>[2x]MRSVASDREVRGPASTEEELSAVLTSIDSSAIASNIQHHADFTPLFSPEHSSPLKAYHATAKSVFDSLIMNWNATYDYYNKVNAKQAYYLSMEFLQGRALTNAIGNLELTGQYAEALKQLGHNLEDVASQEPDPALGNGGLGRLASCFLDSLATLNYPAWGYGLRYRYGLFKQIITKDGQEEVAENWLEMGNPWEIVRNDVSYPVKFYGKVVEGTDGRKHWIGGENIKAVAHDVPIPGYKTKTTNNLRLWSTTVPSQNFDLGA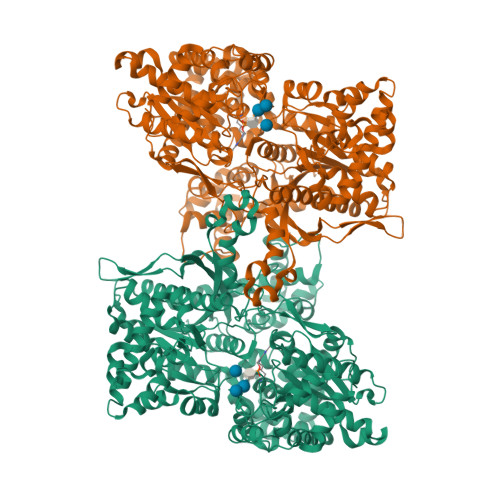FNAGDHAKANEAHLNAEKICHVLYPGDESSEGKILRLKQQYTLCSASLQDIISRFESRAGDSLNWEDFPSKVAVQMNDTHPTLCIPELMRILMDIKGLSWNEAWSITERTVAYTNHTVLPEALEKWSLDIMQKLLPRHVEIIETIDEELMNNIVSKYGTADISLLKQKLKDMRILDNVDLPASVAKLFIKPKEKRGKLLVESLESIAEADEKTESQEVENILSETTEKKAESDSEEAPDAEKEDPEYELDPFAKYDPQFPRVVRMANLCVVGGHSVNGVAEIHSEIVKQDVFNSFYEMWPTKFQNKTNGVTPRRWIRFCNPELSTIISKWIGSDDWILNTDKLAGLKKFADDEDLQSEWRTAKRNNKMKVVSLIRDKTGYIVSPDAMFDVQVKRIHEYKRQLLNILGIVYRYKKMKEMSAKDRRKSFVPRVCIFGGKAFATYVQAKRIVKFITDVAATVNYDPDIGDLLKVVFVPDYNVSVAETLIPASELSQHISTAGMEASGTSNMKFAMNGCLLIGTLDGANVEIREEVGEENFFLFGAHAPEIAGLRQERAEGKFVPDLRFEEVKEYVRSGVFGTSNYDELMGSLEGNEGYGRADYFLVGKDFPSYIECQEKVDEAYRDQKLWTRMSILNTAGSPKFSSDRTIHEYAKDIWDISPVIMPTFPDIENLYFQG>[2x]ETIEIIKDLFEH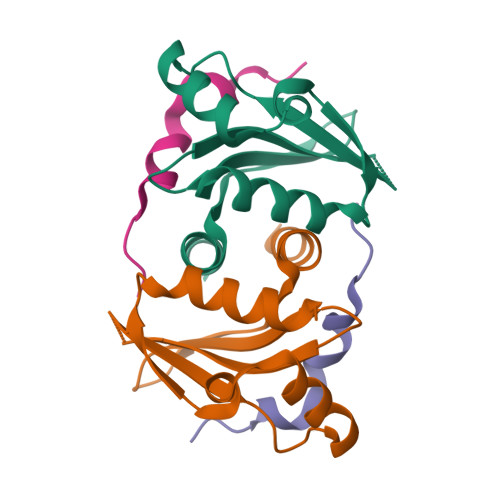LCGVRVHRTYEDDTGLWFDTSQGSKNGIMDYKLGFVKSQAENTTEVDTEVIYVPLLKQRTAEELQELQKKLPDYLFETLSFPLRSLNQFYIKMSKSLNKKV;>[2x]NVQKYIPPTILTKRRNMESFNDCKVNTKDIISFKDVNQEYETWLDKHLSLAKDRD~{N}-(4-morpholin-4-ylthieno[2,3-d]pyrimidin-2-yl)propanamide | C13 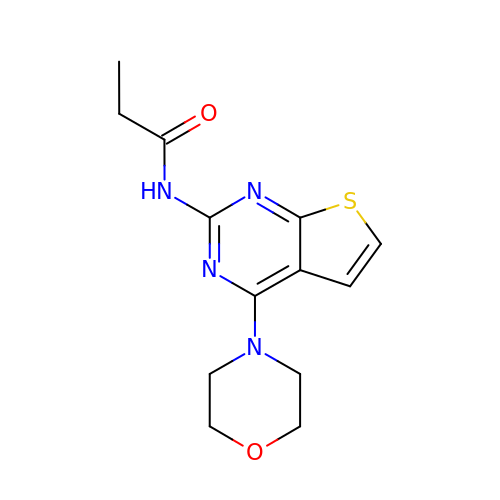H16 N4 O2 S | SJILNVMIBFUZCH-UHFFFAOYSA-N KSHV encoded multifunctional protein ORF57 plays a key role in promoting viral mRNA accumulation and translation. Previous biochemical studies showed that ORF57 is stabilized by dimerization, which is critical for its function. ORF57 comprises of two domains with distinct putative structures: the highly disordered N-terminal domain (NTD) from residue 1 to 166, and the helix-rich C-terminal domain (CTD) from residue 167 to 455. Each monomer contains a zinc ion chelated by four residues, the cysteines at the position 333, 427, 432, and the histidine at 423, which form a consensus zinc-binding motif.

The cubic crystal crystallized at very high concentrations of salt buffer contains 0.01 M MgCl2, 0.05 M HEPES (pH 7.0), 4.0 M LiCl. After data calculation, the cubic crystal consists only of monomers in the crystal asymmetric unit, while in the spindle shape crystal ORF57-CTD forms a dimer in the crystal asymmetric unit and the resolution was relatively lower. As the cubic crystal crystallized in the buffer which has a very high concentration of the salt, it is possible that the dimer was dissolved into monomers by hydrophobic interactions during crystallization. The monomeric crystal belongs to space group I432 and the final structure was refined at resolution of 3.06 Å with R and Rfree values to 22.5% and 26.9%, respectively. The observed monomer structure revealed that ORF57-CTD consists of 11 α-helixes and two short β-sheets. The structure of monomeric ORF57-CTD forms a globular domain which consisting of bundle of 11 α-helixes connected with unstructured loops of various sizes. The N-terminus is represented by an extended “arm” region lacking any α-helixes, but only two unstable small η-helixes (310-helixes). The electron densities for residues V168-R189 and P211-D220 and S455 are not visible in the monomeric structure. The two monomers in the dimeric structure are nearly identical, and the root-mean-square deviation (RMSD) of atomic positions is only 0.528 Å when superimposed, but the N-terminus of the monomeric ORF57-CTD in dimer extends out to a different direction from the N-terminus of monomer if superimposed.

> VSDAVKKLRLPASMIIDGESPRFDDSIIPRHHGACFNVFIPAPPSHVPEVFTDRDITALIRAGGKDDELINKKISAKKIDHLHRQMLSFVTSRHNQAYWVSCRRETAAAGGLQTLGAFVEEQMTWAQTVVRHGGWFDEKDIDIILDTAIFVCNAFVTRFRLLHLSCVFDKQSELALIKQVAYLVAMGNRLVEACNLLGEVKLNFRGGLLLAFVLTIPGMQSRRSISARGQELFRTLLEYYRPGDVMGLLNVIVMEHHSLCRNSECAAATRAAMGSAKFNKGLFFYPLS(1R,3R)-5-[(2Z)-2-[(1R,3aS,7aR)-7a-methyl-1-[(2R)-6-methyl-6-oxidanyl-heptan-2-yl]-2,3,3a,5,6,7-hexahydro-1H-inden-4-ylidene]ethylidene]cyclohexane-1,3-diol 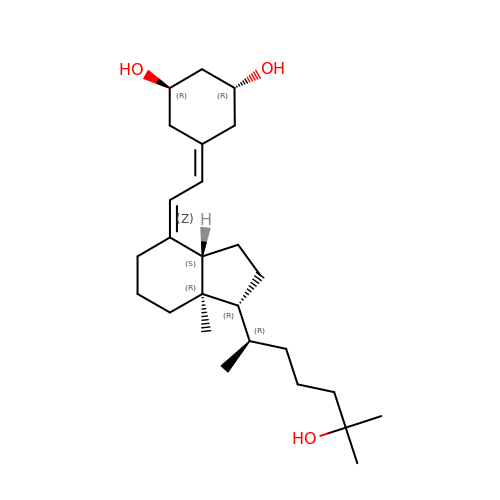| C26 H44 O3 | PKFBWEUIKKCWEW-RXSVZSMJSA-N> MQLSQNVARTTVPSYYHIRTNLPQRKPQNQWEGVYYYSGITKRQQHVVLLQRKREREMYLRQYNRQVASLRGQYAAHHEKPLASLPERLMFATKLASCGMHNEAATFVDAMHHGKELRAIDYVHLISSLRASDLGTCIL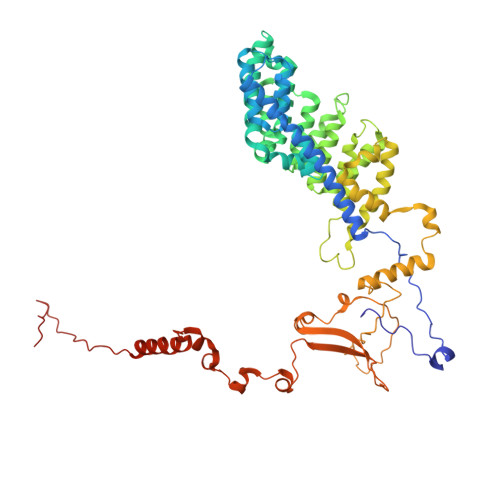HSEAACDPALTFKFLGDNAGAERATEAYRWYDMAMSALAHECGSLRPESTPAASQLTNALMRALMTCGYAHVKAIPDAVYDRMGARGISPTASTYDHVILALALTGNAAEAEDVFRFVRHRHAEHVTVHGYNALLLGNREARLFDRCDGLWQELVDRRWPRANPLTAELYLRSVVDHAYTPTSEGLQRFGSVHVVEKKKVPIVLTQMDELGIPRTHLSGPLRDEVEDALRKFSIYRNRFYEWGRAVKQFDFIEFRRRHGWMYDLHLMKNTTKMLPPIRDPSQPDSTMASAAMVELPAFFTERHPWERNALESLLSVTKERERMDDVRAGDIYYDDTKSIHERSSTWMNEVPETRYDQLYGINHPDVSKIGIRTHLEVEYTNRKEVMEKDAALVRKSIRRGRRLRHRVEVSRTHRNEGSLTAKESK(2E)-2-{2-[4-(4-bromophenyl)-1,3-thiazol-2-yl]hydrazinylidene}-3-(2-nitrophenyl)propanoic acid | C18 H13 Br N4 O4 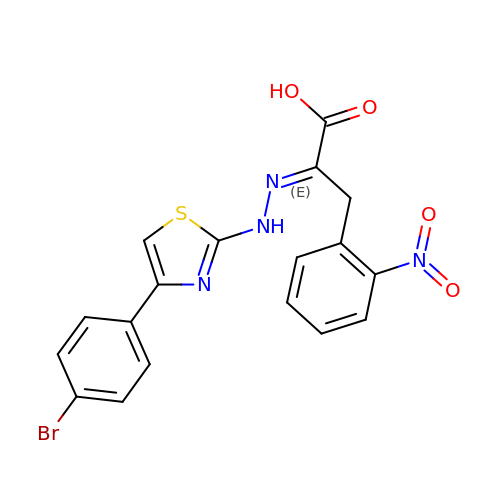S | OHRDQFFRIALSLB-KGENOOAVSA-N> SNAMDTEALANYLLRQLSLDAEENKLEDLLQRQNEDQESSQEYNKKLLLACGFQAILRKILLDARTRATAE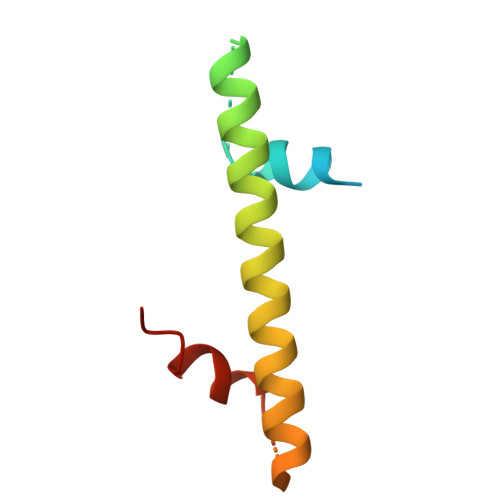GLREVYPYHIEAATQAFLDSQ The isoform GPX4 belongs to a subfamily of selenium-containing GPX enzymes and is unique in that it can also reduce hydroperoxides in complex lipids such as phospho­lipids, cholesterol and cholesteryl ester hydroperoxides, even when they are inserted into biomembranes or lipoproteins. The catalytic mechanism of the GPX reaction involves redox shuttling of this selenocysteine between the redox states selenol (Se–H) and selenenic acid (Se–OH). The catalytic site of GPX enzymes was initially suggested to consist of a catalytic triad formed by a selenocysteine, a glutamine and a tryptophan residue. This was later extended by a conserved asparagine to form a catalytic tetrad, which in human GPX4 consists of Sec46, Gln81, Trp136 and Asn137. Recently, GPX4 has been identified as a key player in ferroptosis, a non-apoptotic cell death resulting from the iron-dependent accumulation of lipid reactive-oxygen species.

To prevent the heterogenous modification observed both with the racemic mixture of ML162 and with the pure enantio­mers, we produced a mutant form of GPX4 in which the second reactive cysteine, Cys66, was mutated to a serine (termed GPX4C66S). Mutation of Cys66 to serine, along with optimization of binding reaction conditions and the use of enantiomerically pure (S)-ML162, enabled the determination of a co-crystal structure at 1.54 Å resolution. The crystal belonged to space group P212121, with one GPX4C66S molecule per asymmetric unit. Clear difference density allowed the building of a complete inhibitor ML162 covalently linked to Sec46. As expected from mass spectrometry, the Cl atom of the inhibitor is lost and the acetamide moiety forms a covalent bond to the Se atom of Sec46. In the absence of a deep binding pocket within the active site of GPX4, it occupies a shallow surface pocket at Sec46 where, in addition to the covalent bond to Sec46, it also forms interactions with the three other residues of the catalytical tetrad (Gln81, Trp136 and Asn137). The side chain of Gln81 adopts a new conformation and rotates away from Sec46, which further enlarges the otherwise very small active site. Surprisingly, the thiophene group of the inhibitor does not engage in any interactions and instead is directed towards the solvent. By interacting with Sec46, Gln81, Trp136 and Asn137, the inhibitor targets all of the residues of the catalytic tetrad of GPX4 and thus fully blocks the active site.

> MCASRDDWRCARSMHEFSAKDIDGHMVNLDKYRGFVCIVTNVASQUGKTEVNYTQLVDLHARYAESGLRILAFPCNQFGKQEPGSNEEIKEFAAGYNVKFDMFSKICVNGDDAHPLWKWMKIQPKGKGILGNAIKWNFTKFLIDKNGCVVKRYGPMEEPLVIEKDLPHYFHHHHHH> MTNAMKVEGYPSMEWPTSLDIPLKASEELVGIDLETDLPDDPTDLKTLLVEENSEKEHWLTIALAYCNHGKTNEGIKLIEMALDVFQNSERASLHTFLTWAHLNLAKGQSLSVETKEHELTQAELNLKDAIGFDPTWIGNMLATVELYYQRGHYDKALETSDLFVKSIHAEDHRSGRQSKPNCLFLLLRAKLLYQKKNYMASLKIFQELLVINPVLQPDPRIGIGLCFWQLKDSKMAIKSWQRALQLNPKNTSASILVLLGEFRESFTNSTNDKTFKEAFTKALSDLNNIFSENQHNPVLLTLLQTYYYFKGDYQTVLDIYHHRILKMSPMIAKIVLSESSFWCGRAHYALGDYRKSFIMFQESLKKNEDNLLAKLGLGQTQIKNNLLEESIITFENLYKTNESLQELNYILGMLYAGKAFDAKTAKNTSAKEQSNLNEKALKYLERYLKLTLATKNQLVISRAYLVISQLYELQNQYKTSLDYLSKALEEMEFIKKEIPLEVLNNLACYHFINGDFIKADDLFKQAKAKVSDKDESVNITLEYNIARTNEKNDCEKSESIYSQVTSLHPAYIAARIRNLYLKFAQSKIEDSDMSTEMNKLLDLNKSDLEIRSFYGWYLKNSKERKNN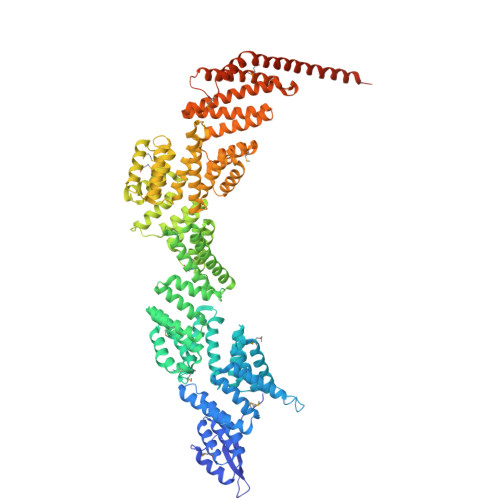EKSTTHNKETLVKYNSHDAYALISLANLYVTIARDGKKSRNPKEQEKSKHSYLKAIQLYQKVLQVDPFNIFAAQGLAIIFAESKRLGPALEILRKVRDSLDNEDVQLNLAHCYLEMREYGKAIENYELVLKKFDNEKTRPHILNLLGRAWYARAIKERSVNFYQKALENAKTALDLFVKESSKSKFIHSVKFNIALLHFQIAETLRRSNPKFRTVQQIKDSLEGLKEGLELFRELNDLKEFNMIPKEELEQRIQLGETTMKSALERSLNEQEEFEKEQSAKIDEARKILEENELKEQGWMKQEEEARRLKLEKQAEEYRKLQDEAQKLIQEREAMAISEHNVKD>[2x]SSPSPLNPGTNVARLAEQAPIHWVSVAQIENSLAGRPPMAVGFDIDDTVLFSSPGFWRGKKTFSPESEDYLKN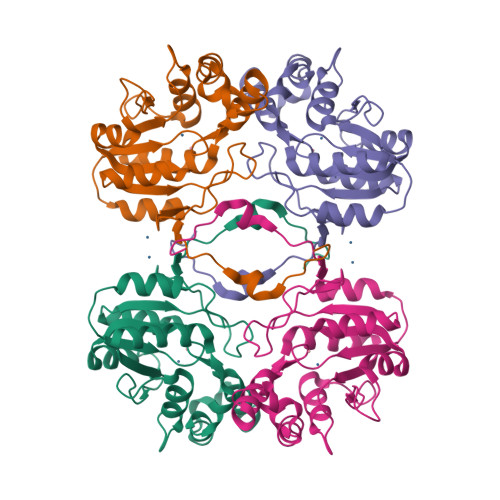PVFWEKMNNGWDEFSIPKEVARQLIDMHVRRGDAIFFVTGRSPTKTETVSKTLADNFHIPATNMNPVIFAGDKPGQNTKSQWLQDKNIRIFYGDSDNDITAARDVGARGIRILRASNSTYKPLPQAGAFGEEVIVNSEY> MSFSGVKVSPECLEAFQELKLGKSLRYVVFKMNDTKTEIVVEKKSTDKDF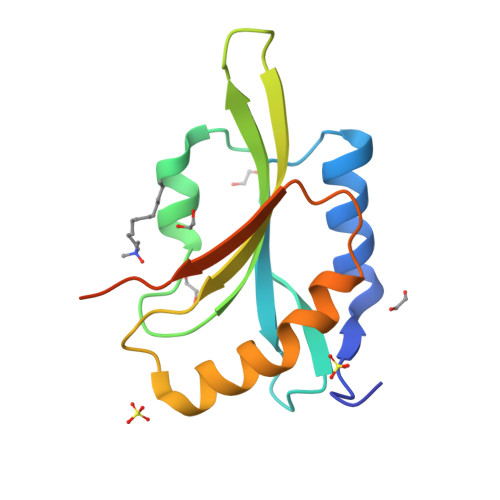DTFLGDLPEKDCRYAIYDFEFNLGEGVRNKIIFISWSPDVAPIKSKMVYSSSKDTLRRAFTGIGTDIQATDFSEVAYETVLEKVTRK>[4x]MLKTNIELKPKVEAFLNEEIKMFINGEFVSAIGGKTFETYNPATEDVLAVVCEAQEEDIDAAVKAARSAFESGPWAEMTTAERAHLIYKLADLIEEHREELAQLEALDNGKPYQVALDDDISATVENYRYY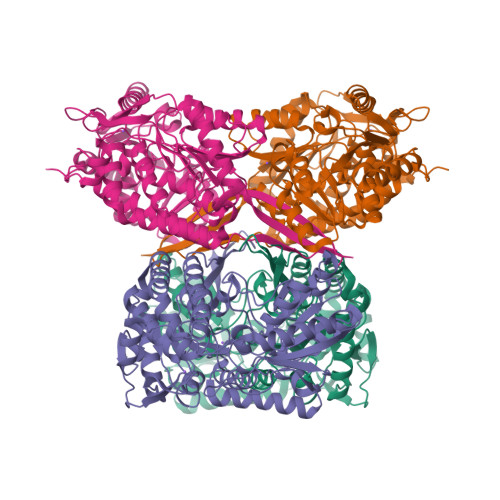AGWTTKIIGQTIPISKDYLNYTRHEPVGVVGQIIPWNFPLVMSSWKMGAALATGCTIVLKPAEQTPLSLLYAAKLFKEAGFPNGVVNFVPGFDPEAGAAIVNHHDIDKVAFTGSTVTGKYIMRQSAEMIKHVTLELGGKSPNIILEDADLEEAINGAFQGIMYNHGQNCSAGSRVFVHRKHYETVVDALVKMANNVKLGAGMEKETEMGPLVSKKQQERVLNYIEQGKKEGATVAAGGERALEKGYFVKPTVFTDVTDDMTIVKEEIFGPVVVVLPFDSTEEVIERANNSSYGLAAGVWTQNIKTGHQVANKLKAGTVWINDYNLENAAAPFGGYKQSGIGRELGSYALDNYTEVKSVWVNIK>GPRARDLGVPFEGTPGALNAITDVAGVEVGHTTVISGDGAMVIGKGPYRTGVTIIHPLGKTSLDGVAAGRAVINGTGEWTGMHLVDEVGQFLGPIALTGTGNVGLVHQSMMDWSVGKVPEEALFSRLLPVVAETLDNRLNDVFGHGLTRDHVFAALDGAKGGPVAEGNVGGGTGMIAYTFKGGIGTSSRVVSAGDTRYTVGVLVQANHGDRNDLRIAGVQIGKEIKGAWPEVNGIVAAGPDAGKPQDKNSLLIVIATDAPLMPHQLERMARRAALGVGRNGSTAGALSGEF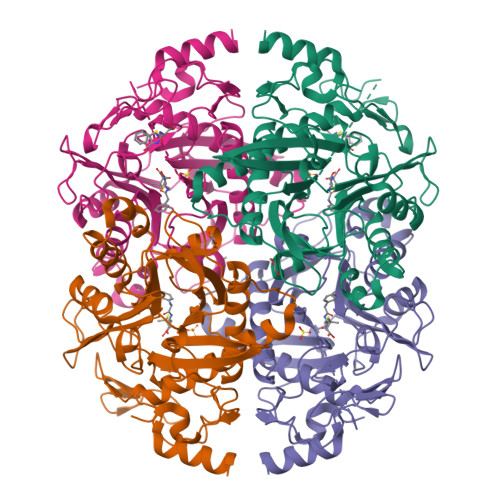ALAFSTSHVIPLGGKPRLPAIINDTDSETMNALFRGVVQATEEALVNQLVASETMTGANNAKVYGIPHDQLARIMKARFPRR[4x]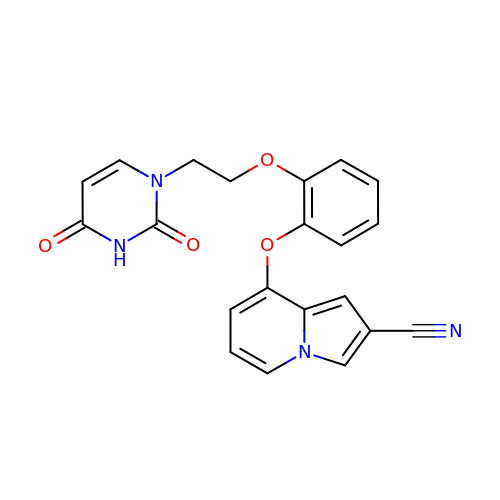8-{2-[2-(2,4-dioxo-3,4-dihydropyrimidin-1(2H)-yl)ethoxy]phenoxy}indolizine-2-carbonitrile | C21 H16 N4 O4 | UUVBMMWJHPNLHN-UHFFFAOYSA-N The Phox homology (PX) domain was first identified in the NADPH phagocyte oxidase complex subunits p40phox and p47phox, and has since been found in proteins in every eukaryotic species from yeast to human. Despite relatively low overall sequence homology, PX domains all possess the same core fold, consisting of three antiparallel β-strands (β1-β3), followed by three α-helices (α1–α3). An extended sequence traverses the protein between helices α1 and α2, termed the PPK loop as it generally contains a conserved ΨPxxPxK motif (Ψ = large aliphatic amino acids V, I, L, and M). Side chains of residues from the β3 strand, α1 helix and PPK loop together form a binding pocket for the headgroup of the canonical lipid PtdIns3P.

We have also obtained two crystal structures of SGK3 and SNX23 (for which previous structures exist), as well as a crystal structure of SNX15, the crystal structure of SNX32 (in complex with a peptide from the bacterial IncE peptide) and the NMR structure of SNX25. The remaining PX domains all bind to a broader range of di- and tri-phosphorylated phosphoinositides. These interactions are shown to arise from the presence of a secondary binding site, centered on a semi-conserved His or Tyr side chain in the α1 helix, associated with nearby positively charged basic side-chains. Interestingly, many of these PX domains show a substantial preference for PtdIns(3,4)P2 (e.g., SNX1, SNX2, SNX22, SGK3, and p47phox), although the functional role of this is not yet clear from our work. When the secondary site is present with an intact canonical binding site then both PtdIns3P and other phosphoinositides can promote membrane association, which will likely contribute to overall membrane avidity.

> GSKESCPSVSIPSSDEHREKKKRFTVYKVLVSVGRSEWFVFRRYAEFDKLYNTLKKQFPAMALKIPAKRIFGDNFDPDFIKQRRAGLNEFIQNLVRYPELYNHPDVRAFLQMDSPKHQ NCgl2760, MSMEG_0317 and Rv0227c, which we collectively term LmcA, lack significant amino-acid sequence similarity to other proteins, making their function difficult to predict. Previously, we identified a new membrane protein, conserved in Corynebacterineae, that is required for synthesis of full-length LM and LAM.

To gain insight into the structure of MSMEG_0317, we focused on the periplasmic domain and produced a truncated form that lacks the predicted signal peptide and transmembrane domain, referred to as MSMEG_0317Δ (residues 30–323), using a M. smegmatis expression system. The N-terminal region folds back and interacts with the C-terminal α-helix located just before the transmembrane domain to form a closed structure that resembles the shape of a ‘cone with a flake’, with the cone being the β-barrel core and the extended α-helix being the flake. All the loops connecting the β-strands and α-turns are ordered except for residues 129–154 within loop 6, which connects β5 and β6. In our MSMEG_0317Δ crystal structure, the electron density of loop 9 is well resolved except for the side chains of Asp226 and Asp227. Loop 9 in this conformation is stabilized by a number of van der Waals interactions, including those of Tyr224 in loop 9 with Gln181 in β7 and of Ala228 in loop 9 with Tyr292 in β14, and a hydrogen-bond interaction between the main chain of Asp229 in loop 9 and the hydroxyl group of Tyr281 in β12.

>[2x]MPEVVFGSTYTKGKIAKIPLDIDTSLVSDGTATAFDPDSLVAERFKIDRDVPVALQQQMSVEAPSNADVVTFQVGTTLRRTDRQQDAGLLLALVDTVTMNRNTAEAVSSENNPGGAVQKPRAIEDEKPPTNIALPHEGLTYRFPFDTEKKTYPFFDPIAQKAFDANYDGEEDVNGLTTYRFVQNVGYDADGKLADPIKYSSLYEDDADASVTARAEVWGVPGEPDESITMDRFYAASRTFWVDPVSGTIVKSEEHGYQYYAREALKPEVTYVDFKVTTNEESVESQVAAASDERDRIALWTRSRHHHHHH> AAEEYTKFPYTIEAEDCDGAGEPWTSVYDTKIKGMYSGKGFAYLTNAPISFNVTVKEDGMYQFTAKVAQILDKGGRLQTISVNGIDYQYTVPYYDTWTDFDFGMHRLNKGANKVSFKPIYGYAEFDTITVEEATFPDFSKVDTKLSDPKATKEAQKLQDYLGSVYGKKIISGQQEIYGGGNDGDYELEFEYIKDLTGKYPAIRGFDFMNYNPLYGWDDQTTERVIEWVKERGGIATASWHINVPKDFDSYELGDKVDWQQCTYATSSTFKTADCIKKGTKENDYWNEAIKMLAEQLQRLQDEKVPLIFRPLHEAEGNVNTDGSGAWFWWGKAGAKTYVEIWKYLYDKLTNEYDLHNLIWEQNLYAWSPDSIQWYAGDEYVDMIGYDK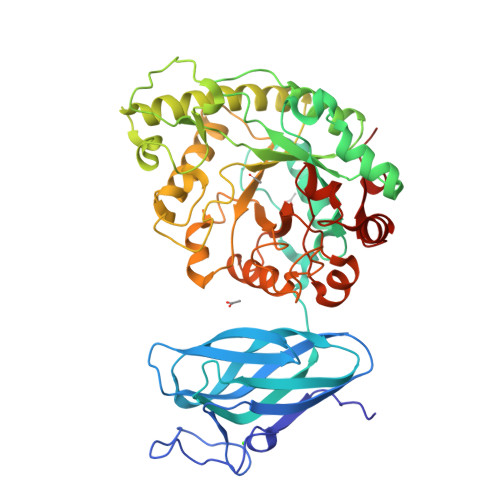YNTVYNRHDGKTSGPNLDAETPIFYTLLNFVENKKMISLAENDSIPGVDNLIIEHAAWLYFCPWYGEFILDEKNNAKSDLKEIYTSDYCITLEDLPFSKKE> MSEGFSSSSIQELYQSLKEITNNADVELFEDRITKLDFESTDEPKHANDIIKDRFLRPSNALPWSLLDMVQDVPHTSSPEDCSGKLDYKELLKVPDPINRTSYQFKRTGLEGKISGYKEEVDLKEVANANASNSLSITRSINHNQNSVRGSTAQLPFTPGGIPMKSVKTDSEQNGSSTMANATKLLHKDGQGLFDIPEGMNRGIKPMDSPAENEDQNGQFKELKQLNEIDNELDIRIEANEAKLKEEEKSAKSISEEIMEEATEETTADNADDAEIDELLPIGIDFGRTKPVSKSVPVKKEWAHVVDLNHKIENFDELIPNPARSWPFELDTFQKEAVYHLEQGDSVFVAAHTSAGKTVVAEYAIAMAHRNMTKTIYTSPIKALSNQKFRDFKETFDDVNIGLITGDVQINPDANCLIMTTEILRSMLYRGADLIRDVEFVIFDEVHYVNDQDRGVVWEEVIIMLPQHVKFILLSATVPNTYEFANWIGRTKQKNIYVISTPKRPVPLEINIWAKKELIPVINQNSEFLEANFRKHKEILNGESAKGAPSKTDNGRGGSTARGGRGGSNTRDGRGGRGNSTRGGANRGGSRGAGAIGSNKRKFFTQDGPSKKTWPEIVNYLRKRELLPMVVFVFSKKRCEEYADWLEGINFCNNKEKSQIHMFIEKSITRLKKEDRDLPQILKTRSLLERGIAVHHGGLLPIVKELIEILFSKGFIKVLFATETFAMGLNLPTRTVIFSSIRKHDGNGLRELTPGEFTQMAGRAGRRGLDSTGTVIVMAYNSPLSIATFKEVTMGVPTRLQSQFRLTYNMILNLLRIEALRVEEMIKYSFSENAKETLQPEHEKQIKVLQEELQTIEYKSCEICDNDIEKFLELMLAYKEATVNLMQEMVKSPSILHILKEGRLVAFRDPNDCLKLGFVFKVSLKDAVCVIMTFTKPYKLPNGEPNHLIYFPKADGYRRRNFPKFQKTDFYMEEVPVTAIEVITKRKFAAPLGKVIKKDVAALNEFNAETNNILDGKTLKEAINIEKQGLKIHQILLDRTNIRDEIFKLKSIKCPNLSQHIVPKFKAHVIKKKIEELYHLMSDQNLSLLPDYEKRLAVLKDTEFIDQNHNVLLKGRVACEINSGYELVLTELILDNFLGSFEPEEIVALLSVFVYEGKTREEEPPIVTPRLAKGKQRIEEIYKKMLCVFNTHQIPLTQDEAEFLDRKRFAMMNVVYEWARGLSFKEIMEMSPEAEGTVVRVITWLDEICREVKTASIIIGNSTLHMKMSRAQELIKRDIVFAASLYL;> GPDSMSDIKQLLKEAKQELTNRDYEETIEISEKVLKLDPDNYFAHIFLGKALSSLPASNNVSSNRNLERATNHYVSAAKLVPDNLLAWKGLFLLFRTTEVVPDILSYDEYFDLCGQYADALLKQEQSQVELINDIKLLKKTHPDCQKAFYQHLKPGSLMAETIGRHLSTPQDALLNLIKILSNIETTEIGKTLSQNRLKLKASDPDYQIKLNSFSWEIIKNSEIDQLYNQLVNILADDQKRSEIENQWLEYRIKVLKSMPLDVKKDFFTKVKEMVEDMVLVNHQSLLAWQKYFEWTDYEDLDNMDAPLIIKYFKKFPKDPLAMILYSWLSSKLSKYDIKSLESANKPPEGHKKTEKETDIKDVDETNEDEVKDRVEDEVKDRVEDEVKDQDEEAKEDEEEDLDDIEIGLLEEEVVTVLTENIVKCKNNILAHRILCQYYLLTKEYEAALPYIKNGISLIAYNIKDLGVHLPLTKREFSLDLATVYTYVDAPKDHNAALKLYDNILSGDFSNIQAKMGKGIIFIERKNWKDAMTLLTQVHEQSPNNLEVLSELSWSKAHMGYMDEALAGLDTVIKGIKGMDLRSIDFRALNLWRQAKVYIMKHASINDAKQENVKCAFKLLIQSIKILDTFAPGFSTLGDIYCHYYKDHLRAFKCYFKAFDLDAGDYTAAKYITETYASKPNWQAASSIASRLIKGEKAKAELRSNNWPFRVVGI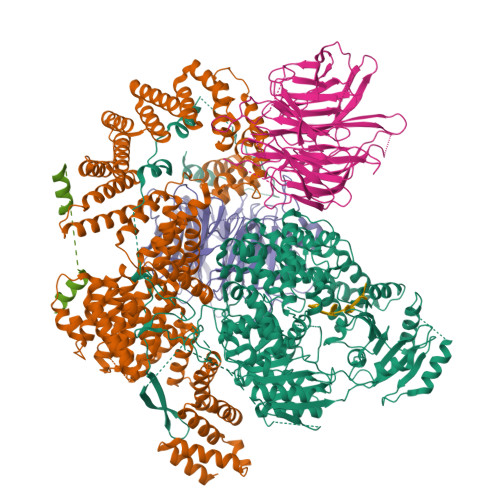AHLEKQEESDSIEWFQSALRVDPNDVESWVGLGQAYHACGRIEASIKVFDKAIQLRPSHTFAQYFKAISLCDVGEYLESLDILEKVCQEAATEESFQIGLVEVLMRCSLDLYSQGFLLKSVSIAKDTIERIKIIISELKCENQQVWIYLSQVLRLFIWIESKVDTLPVESLVSIFENSQFSGSEEIDSVDNIKIDTLLDSTTDDNVSIACKFLILASKYSVSDQKFTDIAGTVRASYWYNIGISELTAFITLKEPQYRDAAIFAFKKSIQLQSNTSETWIGLGIATMDINFRVSQHCFIKATALEPKATNTWFNLAMLGLKKKDTEFAQQVLNKLQSLAPQDSSPWLGMALILEEQGDIIGSSKLFAHSFILSNGRSKAAQFMYAKNVLENHINNGDDERDIETVEKLTTASIALEQFFKKSPDSQFALQCALLTLERLHHYENANELANRLIGILEKKFEKTQDERELFNFAIIKGQFARIHLGLGNFELSIENADLSQGIISESSDEKSMKTKISNHICLGLSYFFLNDFDQTLNQFQELLSISKDSKHLVVLIAKVLYDVGESDTKEIALQELTEYIATSGADLLVTLTIAAMSILDDKREDLSIILEELKALPLSKQIIDKHKDAPYLIEEITKRLYRNDTGKQVWQRSAYFFPNNLKVWERLDKNIQRRIASNGQNKVTAEEMSKLYCESKNLRSIQRGMFLCPWNVTAVKALNECF;>[2x]MSKVFIATANAGKAHDADIFSVSACNSFTVSCSGDGYLKVWDNKLLDNENPKDKSYSHFVHKSGLHHVDVLQAIERDAFELCLVATTSFSGDLLFYRITREDETKKVIFEKLDLLDSDMKKHSFWALKWGASNDRLLSHRLVATDVKGTTYIWKFHPFADESNSLTLNWSPTLELQGTVESPMTPSQFATSVDISERGLIATGFNNGTVQISELSTLRPLYNFESQHSMINNSNSIRSVKFSPQGSLLAIAHDSNSFGCITLYETEFGERIGSLSVPTHSSQASLGEFAHSSWVMSLSFNDSGETLCSAGWDGKLRFWDVKTKERITTLNMHCDDIEIEEDILAVDEHGDSLAEPGVFDVKFLKKGWRSGMGADLNESLCCVCLDRSIRWFREAGGK;> GPDSMSLLEQLARKRIEKSKGLLSADQSHSTSKSASLLERLHKNRETKDNNAETKRKDLKTLLAKDKVKRSDFTPNQHSVSLSLKLSALKKSNSDLEKQGKSVTLDSKENELPTKRKSPDDKLNLEESWKAIKEMNHYCFLKNDPCINQTDDFAFTNFIIKDKKNSLSTSIPLSSQNSSFLSLKKHNNELLGIFVPCNLPKTTRKVAIENFNRPSPDDIIQSAQLNAFNEKLENLNIKSAGSWSHPQFEK> GSHMLSDEQMQIINSLVEAHHKTYDDSYSDFVRFRPPVREGPVTRSASRAASLHSLSDASSDSFNHSPESVDTKLNFSNLLMMYQDSGSPDSSEEDQQSRLSMLPHLADLVSYSIQKVIGFAKMIPGFRDLTAEDQIALLKSSAIEIIMLRSNQSFSLEDMSWSCGGPDFKYCINDVTKAGHTLELLEPLVKFQVGLKKLKLHEEEHVLLMAICLLSPDRPGVQDHVRIEALQDRLCDVLQAYIRIQHPGGRLLYAKMIQKLADLRSLNEEHSKQYRSLSFQPEHSMQLTPLVLEVFGSEVS;> RHKILHRLLQEGSPS

The activities of 1,25D3 are mediated by its binding to the Vitamin D Receptor (VDR, also termed NR1I1), a ligand-dependent transcription factor that belongs to the nuclear receptor superfamily. The 1,25D3 plays a key role in calcium homeostasis by promoting VDR activities in the intestines, bones and kidneys, and is involved in a wide spectrum of biological pathways, including cell differentiation and immune responses. The VDR/RXR heterodimers bind to genomic locations, known as vitamin D response elements (VDRE), within the regulatory regions of their target genes to modulate gene transcription in concert with various co-regulatory molecules. In the present study, by solving the crystal structure of wild type (WT)- and VDRgem-bound to BXL-62, we identify the mechanisms underlying the high potency of the C-20-modified analogs to induce the transcriptional activities of VDR.

To investigate the structural modifications induced by the addition of 16-ene and C-20 cyclopropyl moieties to the 1,25D3 backbone, we determined the crystal structure of the zebrafish (z) VDR LBD in complex with BXL-62. The protein was crystallized in the presence of an excess of BXL-62, and of the human NCoA1 peptide encompassing the second nuclear receptor LXXLL-interacting motif. The structure was solved by molecular replacement and refined to 2.7 Å. BXL-62 adopted a similar orientation in the LBP as 1,25D3, and the BXL-62-bound VDR had the canonical VDR-agonist conformation. Even though the 16-ene moiety reduced the flexibility of the skeleton of 1,25D3, the interactions between VDR and the A-, Seco B-, and C/D- rings of BXL-62 were similar to those of 1,25D3. In addition, the hydroxyl group in C1, C3, and C25 of BXL-62 and of 1,25D3 formed a similar interaction with zSer265 and zArg302, with zTyr175 and zSer306, and with zHis333 and zHis423, respectively. Moreover, all of the contacts identified between zVDR and the 1,25D3 lateral side chain were conserved in the zVDR-BXL-62 complex, as well as the additional interactions with the residues of H6 (zVal328), loop (L) 6–7(zHis333), H7 (zLeu338, zLeu341), and H11 (zHis423) that were formed in the presence of BXL-62. These contacts were induced by the positioning of the side chain, as shown by the torsion angles of C16-C17-C20-C22 (−130° for BXL-62 and -29° for 1,25D3) imposed by the 16-ene configuration and the C-20 cyclopropyl group of BXL-62, resulting in the cyclopropyl pointing towards H7. In addition, the distances between the C25 geminal methyl groups and the C-terminal residues zLeu440 (loop 11–12) and zPhe448 (H12) were reduced in the presence of BXL-62 than in the presence of 1,25D3. Thus, the increased rigidity imposed by the geometry of the 16-ene configuration and of the C-20 cyclopropyl group, as well as the stronger/additional interactions, contribute to a more stable VDR agonist conformation.>[3x]GPMGKPARKGCEWKRFLKNNWVLLSTVAAVVLGITTGVLVREHSNLSTLEKFYFAFPGEILMRMLKLIILPLIISSMITGVAALDSNVSGKIGLRAVVYYFCTTLIAVILGIVLVVSIKPGVTQKVGEIARTGSTPEVSTVDAMLDLIRNMFPENLVQACFQQYKTKREEVKPPSDPEMNMTEESFTAVMTTAISKNKTKEYKIVGMYSDGINVLGLIVFCLVFGLVIGKMGEKGQILVDFFNALSDATMKIVQIIMCYMPLGILFLIAGKIIEVEDWEIFRKLGLYMATVLTGLAIHSIVILPLIYFIVVRKNPFRFAMGMAQALLTALMISSSSATLPVTFRCAEENNQVDKRITRFVLPVGATINM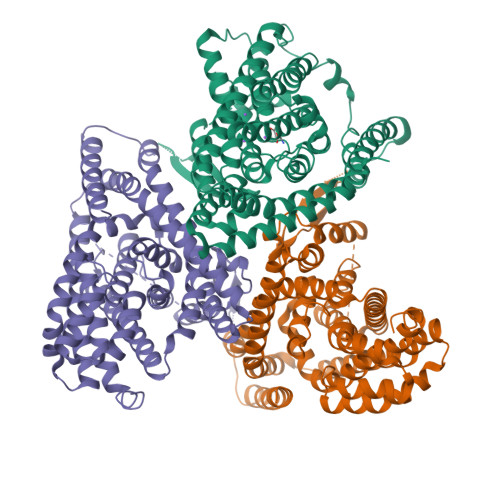DGTALYEAVAAVFIAQLNDLDLGIGQIITISITATSASIGAAGVPQAGLVTMVIVLSAVGLPAEDVTLIIAVDWLLDRFRTMVNVLGDAFGTGIVEKLSKKELEQMDVSSEVNIVNPFALESTILDNEDSDTKKSYVNGGFAVDKSDTISFTQTSQF2-HYDROXYETHYL 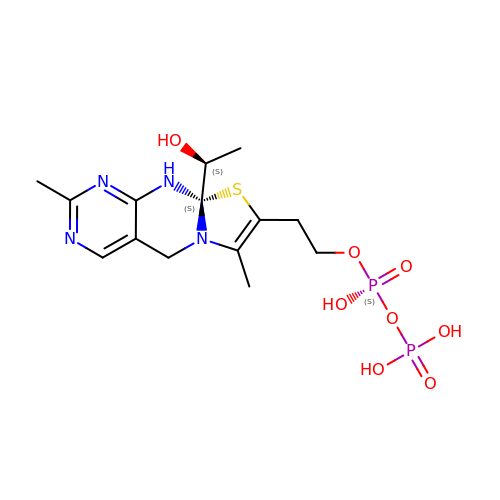DIHYDROTHIACHROME DIPHOSPHATE | C14 H22 N4 O8 P2 S | UQFVHIGKDHNMJT-XPTSAGLGSA-N>ANPCCSNPCQNRGECMSTGFDQYKCDCTRTGFYGENCTTPEFLTRIKLLLKPTPNTVHYILTHFKGVWNIVNNIPFLRSLIMKYVLTSRSYLIDSPPTYNVHYGYKSWEAFSNLSYYTRALPPVADDCPTPMGVKGNKELPDSKEVLEKVLLRREFIPDPQGSNMMFAFFAQHFTHQFFKTDHKRGPGFTRGLGHGVDLNHIYGETLDRQHKLRLFKDGKLKYQVIGGEVYPPTVKDTQVEMIYPPHIPENLQFAVGQEVFGLVPGLMMYATIWLREHQRVCDILKQEHPEWGDEQLFQTSKLILIGETIKIVIEDYVQHLSGYHFKLKFDPELLFNQQFQYQNRIASEFNTLYHWHPLLPDTFNIEDQEYSFKQFLYNNSILLEHGLTQFVE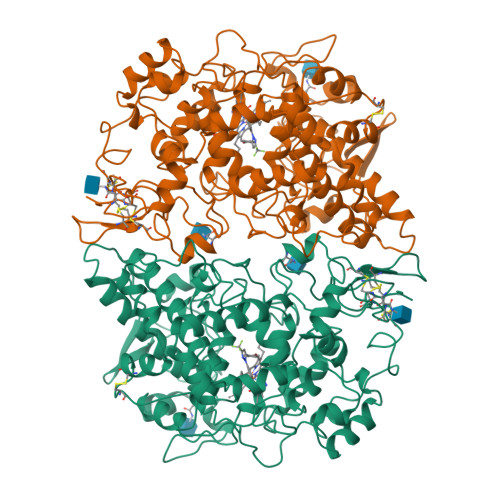SFTRQIAGRVAGGRNVPIAVQAVAKASIDQSREMKYQSLNEYRKRFSLKPYTSFEELTGEKEMAAELKALYSDIDVMELYPALLVEKPRPDAIFGETMVELGAPFSLKGLMGNPICSPQYWKPSTFGGEVGFKIINTASIQSLICNNVKGCPFTSFNVQDPQPTKTATINASASHSRLDDINPTVLIKRRSTEL[4x]> MSVYKGGVDCPLVVKLYATVGLHRYNMLEGTNLYLHKIEKYVVVCTLMPVSYNITLIAEDPATSSFVVFETNVDQRSLGQIDF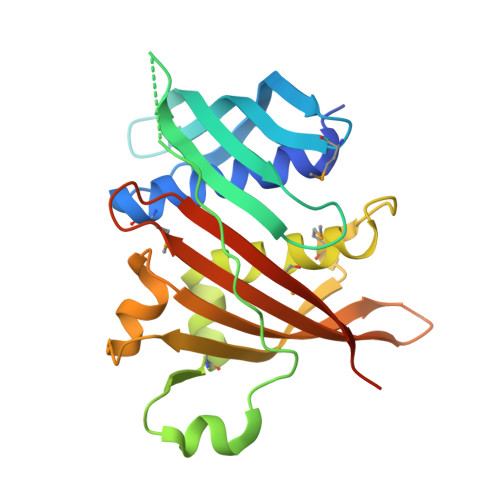TCYISRPKGIKSEIYPNQFFDAKDLPDKWPSKEAFADQSRFLYKMQKSDWEEHDWIRLYMEISFFNRDRCLDHNMSDLKILDVVVETEENVPRETVLKSLRNVLVYIRYDQDLGADGVCKHIAIVRRTVEPTTHCVCLLGESQLVPDSELEHHHHHHHH> MYKLLKVKDVVRIPPRMFTMDPKEAAKIVLRETYEGIYDRDEGVVLAILDVEEISEGVIVPGDGATYHEAIFNVLVWEPR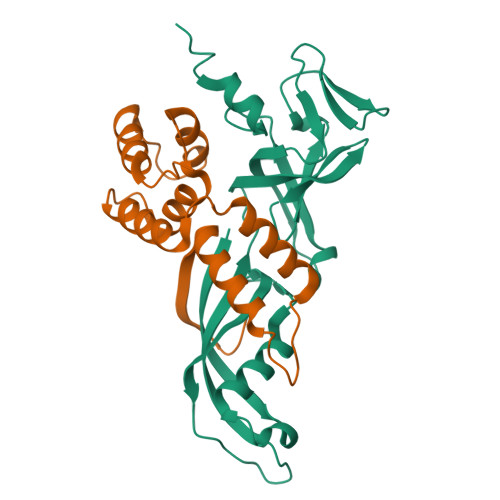NQEVVEGEVVEMMPYGAFIRIGPMDGLVHISQLMDDYVVFDEKNRQFIGKETNRVLKLGDYVRARIIGVSVKSRVIRENKINMTMRQPGLGKFEWIEKEKKKAKEESKGE;> MIGRKKLEEHYITIAEAKELLERRHAEGLAENPEEPMFYEARVSLEHAERFAKLKPEQARELKEKLMGLFDWINERIAAKLVDILPEDYLDIRVIFAKEEYMPTPEEAEEIIKVIDEYRPLE> SMAHGGLQRGNKKIPESSNVGGSRK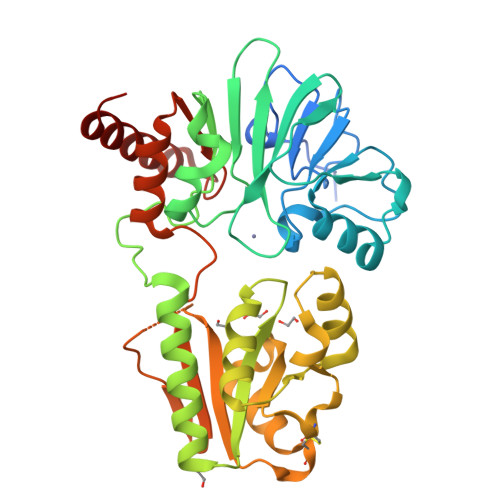KTCPFYKKIPGTGFTVDAFQYGVVEGCTAYFLTHFHSDHYAGLSKHFTFPVYCSEITGNLLKNKLHVQEQYIHPLPLDTECIVNGVKVVLLDANHCPGAVMILFYLPNGTVILHTGDFRADPSMERSLLADQKVHMLYLDTTYCSPEYTFPSQQEVIRFAINTAFEAVTLNPHALVVCGTYSIGKEKVFLAIADVLGSKVGMSQEKYKTLQCLNIPEINSLITTDMCSSLVHLLPMMQINFKGLQSHLKKCGGKYNQILAFRPTGWTHSNKFTRIADVIPQTKGNISIYGIPYSEHSSYLEMKRFVQWLKPQKIIPTVNVGTWKSRSTMEKYFREWKLEAGY N-{4-[1-(2-methylpropanoyl)piperidin-4-yl]phenyl}-2H-pyrrolo[3,4-c]pyridine-2-carboxamide | C23 H26 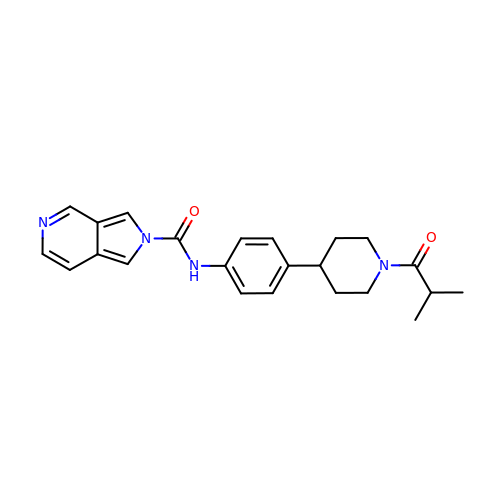N4 O2 | UXDAQOSAZJARDY-UHFFFAOYSA-N> MSGIALSRLAQERKAWRKDHPFGFVAVPTKNPDGTMNLMNWECAIPGKKGTPWEGGLFKLRMLFKDDYPSSPPKCKFEPPLFHPNVYPSGTVCLSILEEDKDWRPAITIKQILLGIQELLNEPNIQDPAQAEAYTIYCQNRVEYEKRVRAQAKKFAPS;> MEYIKLKVIGQDSSEIHFK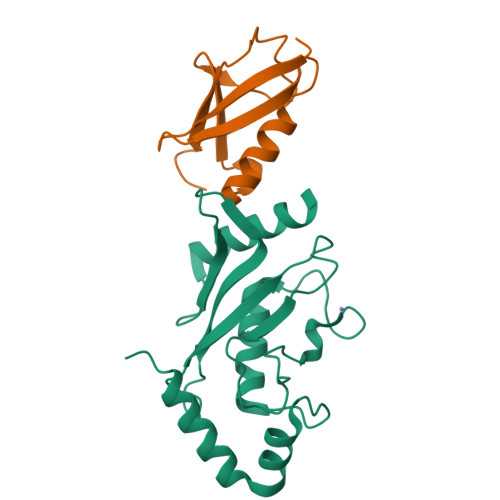VKMTTHLKKLKESYCQRQGVPMNSLRFLFEGQRIADNHTPKELGMEEEDVIEVYQEQTGG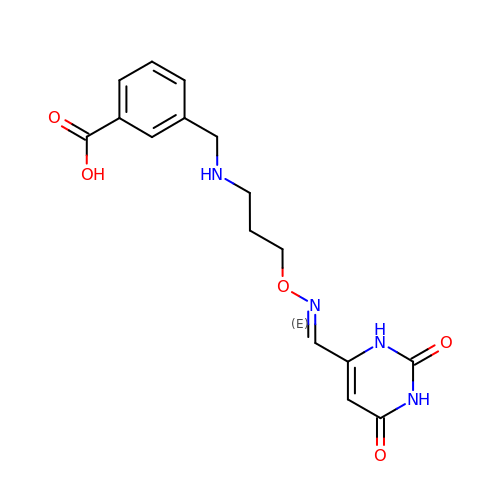3-({[3-({[(1E)-(2,6-dioxo-1,2,3,6-tetrahydropyrimidin-4-yl)methylidene]amino}oxy)propyl]amino}methyl)benzoic acid | C16 H18 N4 O5 | CZTGLADCGFOCLD-VCHYOVAHSA-N>[5x]PQPCLTGPRTCKDLLDRGHFLSGWHTIYLPDCRPLTVLCDMDTDGGGWTVFQRRVDGSVDFYRDWATYKQGFGSRL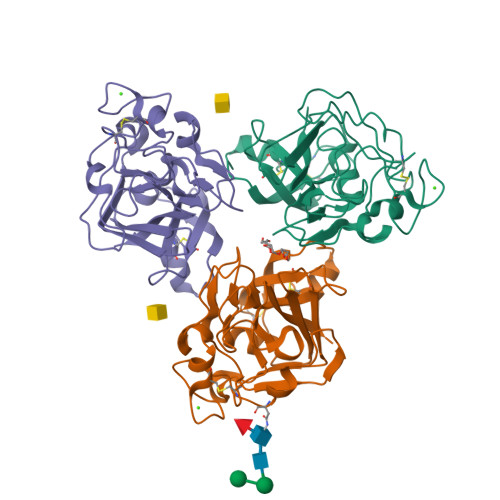GEFWLGNDNIHALTAQGTSELRTDLVDFEDNYQFAKYRSFKVADEAEKYNLVLGAFVEGSAGDSLTFHNNQSFSTKDQDNDLNTGNCAVMFQGAWWYKNCHTSNLNGRYLRGTHGSFANGINWKSGKGYNYSYKVSEMKVRPA;> PQPCLTGPRTCKDLLDRGHFLSGWHTIYLPDCRPLTVLCDMDTDGGGWTVFQRRVDGSVDFYRDWATYKQGFGSRLGEFWLGNDNIHALTAQGTSELRTDLVDFEDNYQFAKYRSFKVADEAEKYNLVLGAFVEGSAGDSLTFHNNQSFSTKDQDNDLNNGNCAVMFQGAWWYKNCHTSNLNGRYLRGTHGSFANGINWKSGKGYNYSYKVSEMKVRPA> SNAADFRTYRAEKNYAVNSGKWYFEFEILTAGPMRVGWAHADMPPGMMLGQDENSWAFDGYNEEKVYVNSSESFGKQWAVGDVVGVFLDLIDNTISFSLNGELLMDALGGETTFADVQGDNFVPACTLGVGQKARLTYGQD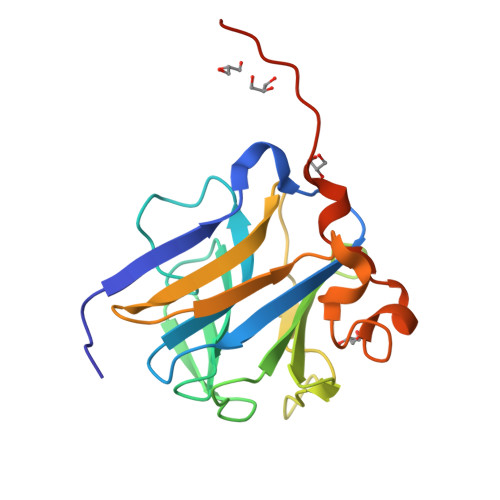VNTLKYFTTCGLQEGYEPFCVNMARDVTHWYTKDQPIFE>ALLQKTRIINSMLQAAAGKPVNFKEMAETLRDVIDSNIFVVSRRGKLLGYSINQQIENDRMKKMLEDRQFPEEYTKNLFNVPETSSNLDINSEYTAFPVENRDLFQAGLTTIVPIIGGGERLGTLILSRLQDQFNDDDLILA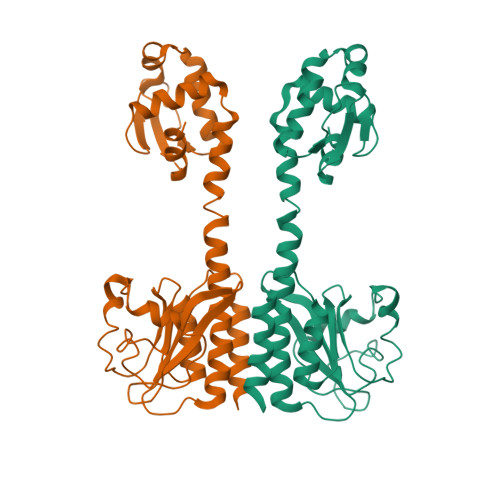EYGATVVGMEILREKAEEIEEEARSKAVVQMAISSLSYSELEAIEHIFEELDGNEGLLVASKIADRVGITRSVIVNALRKLESAGVIESRSLGMKGTYIKVLNNKFLIELENLKSHHHHHH[2x]[(2R,3S,4R,5R)-5-(6-amino-8-bromo-9H-purin-9-yl)-3,4-dihydroxytetrahydrofuran-2-yl]methyl [(2R,3S,4S)-3,4-dihydroxytetrahydrofuran-2-yl]methyl dihydrogen diphosphate | C15 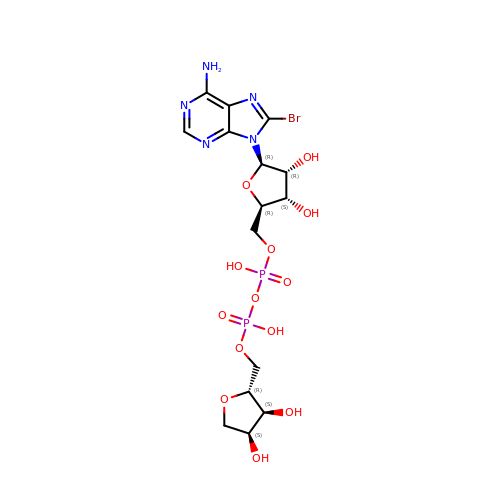H22 Br N5 O13 P2 | DTBPYRLOWSYQCZ-ZVIMGNLFSA-L>[2x]MTTS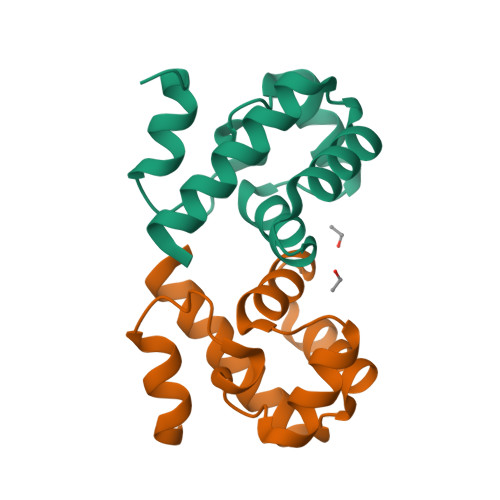QKHRDFVAEPMGEKPVGSLAGIGEVLGKKLEERGFDKAYVVLGQFLVLKKDEDLFREWLKDTCGANAKQSRDCFGCLREWCDAFL>[8x]GAGAMSSRKKPSRRTRVLVGGAALAVLGAGVVGTVAANAADTTEATPAAAPVAARGGELTQSTHLTLEAAT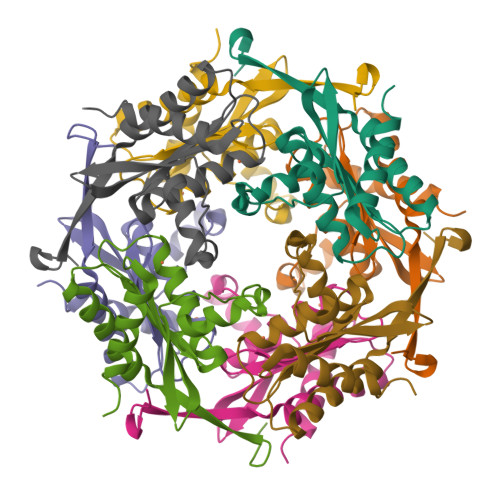KAARAAVEAAEKDGRHVSVAVVDRNGNTLVTLRGDGAGPQSYESAERKAFTAVSWNAPTSELAKRLAQAPTLKDIPGTLFLAGGTPVTAKGAPVAGIGVAGAPSGDLDEQYARAGAAVLGH(4R)-3-(4-[4-(2-chlorophenyl)piperazin-1-yl]-6-{[2-methyl-6-(methylcarbamoyl)phenyl]amino}-1,3,5-triazin-2-yl)-N-methyl-1,3-thiazolidine-4-carboxamide 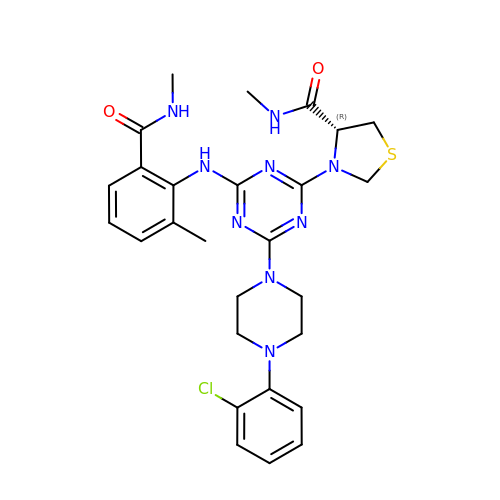| C27 H32 Cl N9 O2 S | QRGGVLXBPSQEDF-NRFANRHFSA-N>MADLAESNIKVMCRFRPLNESEVNRGDKYIAKFQGEDTVVIASKPYAFDRVFQSSTSQEQVYNDAAKKIVKDVLEGYNGTIFAYGQTSSGKVHTMEGKLHDPEGMGIIPRIVQDIFNYIYSMDENLEFHIKVSYFEIYLDKIRDLLDVSKTNLSVHEDKNRVPYVKGATERFVSSPDEVMDTIDEGKSNRHVAVTNMNEHSSRSHSIFLINVKQENTQTEQKLSGKLYLVDLAGSEKVSKTGAEGAVLDEAKNINKSLSALGNVISALAEGSTYVPYRDSKMTRILQDSLGGNARTTIVICCSPSSYNESETKSTLLFGQRA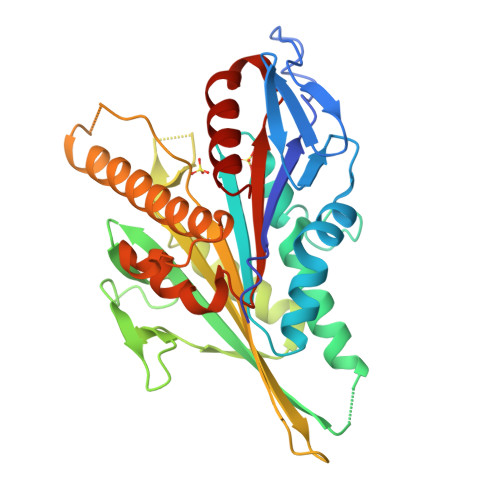KTI[6x]> MSDMNNPSDENTGALDDLWADALNEQKATTTKSAADAVFQQLGGGDVSGAMQDIDLIMDIPVKLTVELGRTRMTIKELLRLTQGSVVALDGLAGEPLDILINGYLIAQGEVVVVADKYGVRITDIIT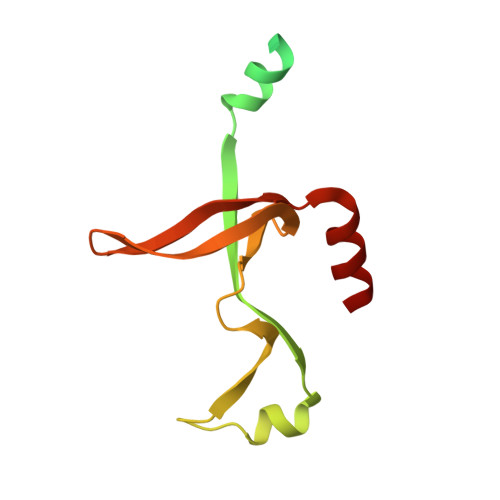PSERMRRLSR> GANNLVETTCKNTPNYQLCLKTLLSDKRSATGDITTLALIMVDAIKAKANQAAVTISKLRHSNPPAAWKGPLKNCAFSYKVILTASLPEAIEALTKGDPKFAEDGMVGSSGDAQECEEYFKGSKSPFSALNIAVHELSDVGRAI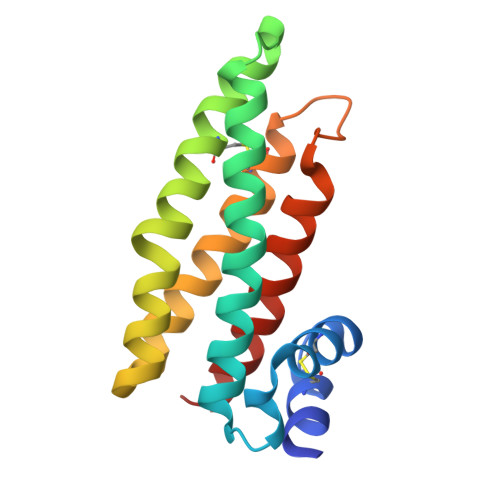VRNLL>MGAAPDSHQLAKALAEAADVGAQMIKLVGLRELSEAERQLRSLVVALMQEVFTEFFPGCVVHPFGSSINSFDVHGCDLDLFLDL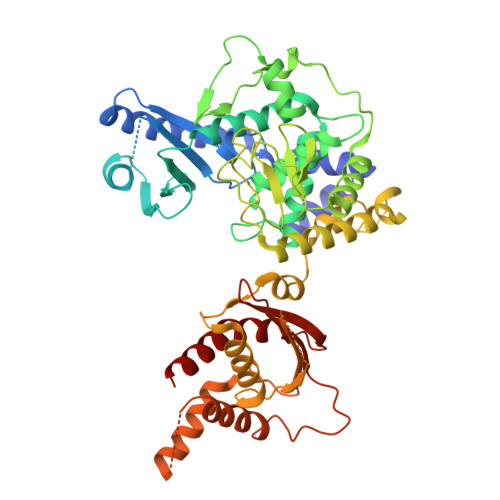GDLEEPQPVPKLPPASPLLEDREEGDLGKASELAETPKEEKAEGAAMLELVGSILRGCVPGVYRVQTVPSARRPVVKFCHRPSGLHGDVSLSNRLALHNSRFLSLCSELDGRVRPLVYTLRCWAQGRGLSGSGPLLSNYALTLLVIYFLQTRDPPVLPTVSQLTQKAGEGEQVEVDGWDCSFPRDASRLEPSINVEPLSSLLAQFFSAVSSWDLRGSLLSLREGQALPVAGGLPSNLWEGLRLGPLNLQDPFDLSHNVAANVTSRVAGRLQNCCRAAANYCRSLQYQRRSSRGRDWGLLPLLQPSSPSSLLSATPIPLPLAPFTQLTAALVQVFREALGCHIEQATKRTRSEGGGTGQGEAGKGASLPSSASWRCALWHRVWQGRRRARRRLQQQTKEGAGGGAGTRAGWLATEAQVTQELKGLSGGEERPETEPLLSFVASVSPADRMLTVTPLQDPQGLFPDLHHFLQVFLPQAIRHLKLEHHHHHH[4x]> MRGSAFNGKWETESQEGYEPFCKLIGIPDDVIAKGRDFKLVTEIVQNGDDFTWTQYYPNNHVVTNKFIVGKESDMETVGGKKFKGIVSMEGGKL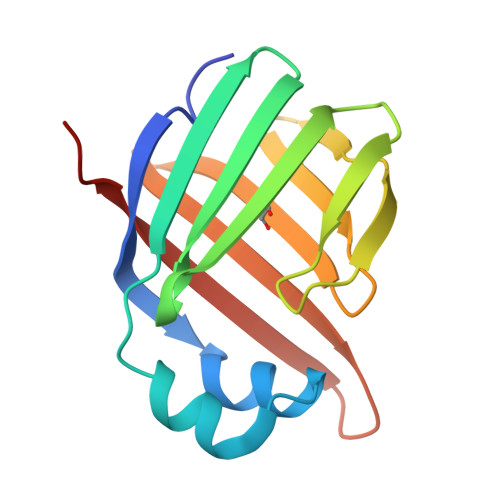TISFPKYQQTTEISGGKLVETSTASGAQGTAVLVRTSKKVLVPR The fungal Bromodomain and Extra‐Terminal (BET) protein Bdf1 is a potential antifungal target against invasive fungal infections. One attractive target is the fungal BET protein Bdf1, a global transcriptional regulator. BET proteins bind chromatin through their two bromodomains (BDs), BD1 and BD2, which specifically recognize histones acetylated on lysines. We show that Bdf1 is essential in C. glabrata, and that inactivation of both Bdf1 BDs induces lethality.

We adapted our HTRF assay to perform a high‐throughput (HT) screen of small molecule inhibitors selective for CgBdf1 BDs over human BET BDs. We repurchased and rescreened these compounds and subsequently tested the 12 most potent hits against CgBD1 and CgBD2 and the corresponding human Brd4 BDs. This revealed 4 non‐selective inhibitors active against all four BDs and 8 compounds selective for CgBD1. To better understand the different selectivities of these compounds, we determined BD co‐crystal structures for the non‐selective tetrahydropyridoindole 29 and the CgBD1‐selective methylpyrazole 63. The structure of 29 bound to CgBD2 shows that the compound's acetyl group forms direct and water‐mediated H bonds with Asn386 and Tyr343 in the BC and ZA loops, respectively, while the morpholinylphenyl moiety packs against Tyr327 in its gauche− conformation. Structural alignments reveal that the binding pockets of CgBD1 and of Brd4 BD1 and BD2 can all accommodate 29, explaining its poor selectivity.

> AMGQRAMKFCQGVVRELMSKKYASFNYPFLEPVDPVALNCPTYFDYVKEPMDLGTVSKKLSNWEYENLDQAEHDIRLIFQNCYAFNPDGTIVNMMGHRLEDIFNTKWADRPLYSDVES In this context, the highly active, efficient, and selective metal-dependent Formate Dehydrogenases (Fdh) are very appealing systems that enable harnessing millions of years of natural evolution. Additionally, [4Fe–4S] clusters are present to convey electrons to/from the physiological partners. Additionally, the oxygen sensitivity of these enzymes must also be understood as it poses an important obstacle for biotechnological applications. This work presents a combined biochemical, spectroscopic, and structural characterization of Desulfovibrio vulgaris FdhAB (DvFdhAB) when exposed to oxygen in the presence of a substrate (formate or CO2).

To study the effect of O2 in the presence of the CO2 substrate, High Pressure (HP) gas soaking experiments were performed at the HP Macromolecular Crystallography Lab (HPMX, ESRF, Grenoble, France). Unexpectedly, crystals from the aerobically isolated oxidized form (prepared in the absence of formate) pressurized with 48 bar of CO2 in aerobic conditions resulted in a structure (HP_CO2) nearly identical to the Reox_120 min structure (Table S1†). The HP_CO2 structure shows the same SeCys dissociated form as well as clear electron density for a dioxygen/peroxide molecule coordinated to the W ion. These data show unequivocally that exposure to oxygen in the presence of either substrate results in the W–OO⋯SeCys dissociated form, and that, contrary to previous reports, tungsten reduction is not a pre-requisite for enzyme inactivation. Remarkably, a CO2 molecule is present near the active site, which has never been observed before. The CO2 molecule is found close to the W centre (4.3 Å away) and the catalytic SeCys (4.0 Å away), being stabilized by van der Waals contacts with the carbonyl of L440 and with the dioxygen ligand, plus a hydrogen bonding interaction to the NH of G442. Although the inactive form of the enzyme was captured, the location of the CO2 molecule may represent a transient affinity position along the CO2 diffusion pathway from the solvent to the active site, as suggested by Laun et al., 2022,30 for the Fdh from R. capsulatus. This is further supported by the increased B-factor of the CO2 molecule (∼50 Å2), when compared with the B-factors of the neighbouring backbone (∼25 Å2) and sidechains (∼30 Å2). Since the SeCys dissociated form was also obtained with exposure to oxygen in the presence of CO2 (HP_CO2), the activity of DvFdhAB was also monitored in these conditions. In fact, co-exposure of a solution of non-activated DvFdhAB to oxygen and CO2 led to 80% loss of activity in 30 min, whereas full inactivation of the DTT-activated enzyme occurs in 30 minutes, or less.

> MTVTRRHFLKLSAGAAVAGAFTGLGLSLAPTVARAELQKLQWAKQTTSICCYCAVGCGLIVHTAKDGQGRAVNVEGDPDHPINEGSLCPKGASIFQLGENDQRGTQPLYRAPFSDTWKPVTWDFALTEIAKRIKKTRDASFTEKNAAGDLVNRTEAIASFGSAAMDNEECWAYGNILRSLGLVYIEHQARIUHSPTVPALAESFGRGAMTNHWNDLANSDCILIMGSNAAENHPIAFKWVLRAKDKGATLIHVDPRFTRTSARCDVYAPIRSGADIPFLGGLIKYILDNKLYFTDYVREYTNASLIVGEKFSFKDGLFSGYDAANKKYDKSMWAFELDANGVPKRDPALKHPRCVINLLKKHYERYNLDKVAAITGTSKEQLQQVYKAYAATGKPDKAGTIMYAMGWTQHSVGVQNIRAMAMIQLLLGNIGVAGGGVNALRGESNVQGSTDQGLLAHIWPGYNPVPNSKAATLELYNAATPQSKDPMSVNWWQNRPKYVASYLKALYPDEEPAAAYDYLPRIDAGRKLTDYFWLNIFEKMDKGEFKGLFAWGMNPACGGANANKNRKAMGKLEWLVNVNLFENETSSFWKGPGMNPAEIGTEVFFLPCCVSIEKEGSVANSGRWMQWRYRGPKPYAETKPDGDIMLDMFKKVRELYAKEGGAYPAPIAKLNIADWEEHNEFSPTKVAKLMNGYFLKDTEVGGKQFKKGQQVPSFAFLTADGSTCSGNWLHAGSFTDAGNLMARRDKTQTPEQARIGLFPNWSFCWPVNRRILYNRASVDKTGKPWNPAKAVIEWKDGKWVGDVVDGGGDPGTKHPFIMQTHGFGALYGPGREEGPFPEHYEPLECPVSKNPFSKQLHNPVAFQIEGEKKAVCDPRYPFIGTTYRVTEHWQTGLMTRRCAWLVEAEPQIFCEISKELAKLRGIGNGDTVKVSSLRGALEAVAIVTERIRPFKIEGVDVHMVGLPWHYGWMVPKNGGDTANLLTPSAGDPNTGIPETKAFMVDVRKVWSHPQFEK;> MGKMFFVDLSRCTACRGCQIACKQWKNLPAEETRNTGSHQNPPDLSYVTLKTVRFTEKSRKGPGIDWLFFPEQCRHCVEPPCKGQADVDLEGAVVKDETTGAVLFTELTAKVDGESVRSACPYDIPRIDPVTKRLSKCDMCNDRVQNGLLPACVKTCPTGTMNFGDEQEMLALAEKRLAEVKKTYPGAVLGDPNDVRVVYLFTRDPKDFYEHAVA>EGDIHMKKGHHHHHHENLYFQGGSGKLSEQLKHCNGILKELLSKKHAAYAWPFYKPVDASALGLHDYHDIIKHPMDLSTVKRKMENRDYRDAQEFAADVRLMFSNCYKYN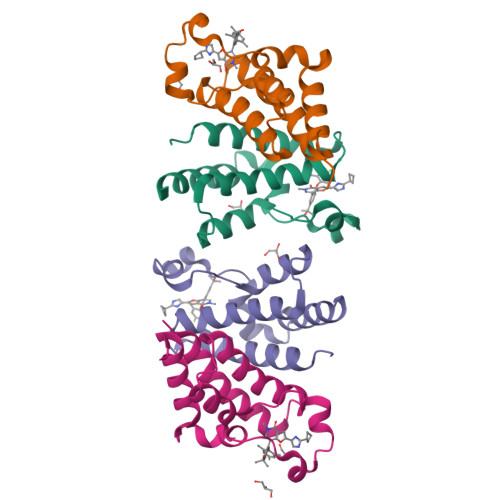PPDHDVVAMARKLQDVFEFRYAKMPD[4x]> MAQSKGSVDQTLHAPHCEVGCAANVARRVGVDLARQVIGAHWASRMLVREVGTFPQPLLDRTQVTFSAQGEGWPALLARMTGGEVTSRHVPREELLSTLHADRAEGGTLLFMEDRACPWLDSAHSPGMLPHVVVPDGVAPDGSWQLIEGHSWWRGRYAMSEQDLLAASYPDPDPHHVAGRVLSLRIRPSAERAAQLDTLARQELAAGLRTYLAAEC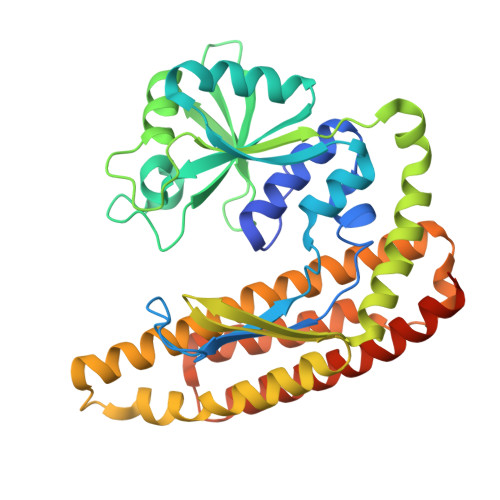GETETPAGRIVWANGPQSVPLLVERLRGWDYLCPLAARNDLSTEHARDVALGRYLFLALTDELAFAAYARAGTLRLVEGLGLAGAVGGLRPDEAWRLAWRSGQKLYRRLDRQNLSALFSALEKAAEVDVEYARRLLKELKLAAALEHHHHHHHH> SNAGKKSRVKTQKSGTGATATVSPKEILNLTSELLQKCSSPAPGPGKEWEEYVQIRTLVEKIRKKQKGLSVTFDGKREDYFPDLMKWASENGASVEGFEMVNFKEEGF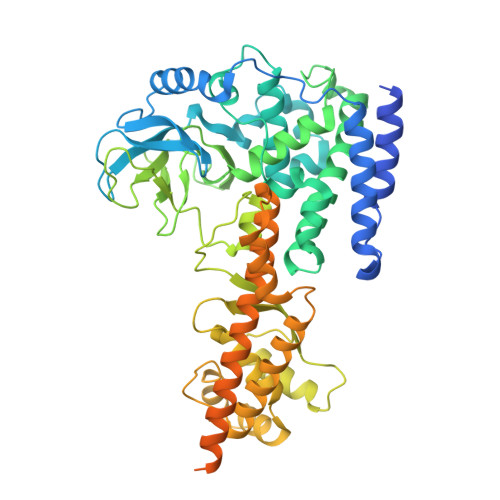GLRATRDIKAEELFLWVPRKLLMTVESAKNSVLGPLYSQDRILQAMGNIALAFHLLCERASPNSFWQPYIQTLPSEYDTPLYFEEDEVRYLQSTQAIHDVFSQYKNTARQYAYFYKVIQTHPHANKLPLKDSFTYEDYRWAVSSVMTRQNQIPTEDGSRVTLALIPLWDMCNHTNGLITTGYNLEDDRCECVALQDFRAGEQIYIFYGTRSNAEFVIHSGFFFDNNSHDRVKIKLGVSKSDRLYAMKAEVLARAGIPTSSVFALHFTEPPISAQLLAFLRVFCMTEEELKEHLLGDSAIDRIFTLGNSEFPVSWDNEVKLWTFLEDRASLLLKTYKTTIEEDKSVLKNHDLSVRAKMAIKLRLGEKEILEKAVKSAAVNREYYRQQMEEKAPLPKYEESNLGLLESSVGDSRLPLVLRNLEEEAGVQDALNIREAISKAKATENGLVNGENSIPNGTRSENESLNQESKRAVEDAKGSSSDSTAGVKE> MAIGEFMVSLPRMVYPQPKVLTPCRKDVLVVTPWLAPIVWEGTFNIDILNEQFRLQNTTIGLTVFAIKKYVAFLKLFLETAEKHFMVGHRVHYYVFTDQPAAVPRVTLGTGRQLSVLEVRAYKRWQDVSMRRMEMIS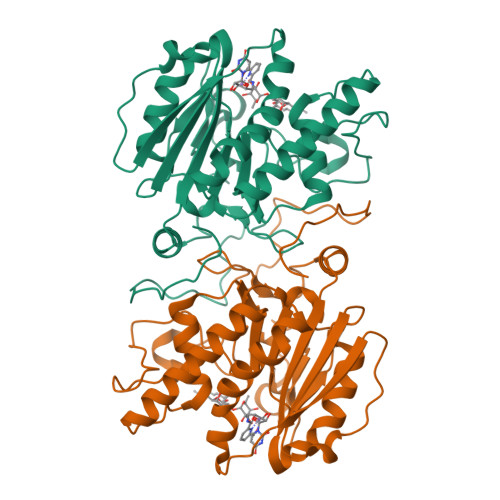DFCERRFLSEVDYLVCVDVDMEFRDHVGVEILTPLFGTLHPGFYGSSREAFTYERRPQSQAYIPKDEGDFYYGGAFFGGSVQEVQRLTRACHQAMMVDQANGIEAVWHDESHLNKYLLRHKPTKVLSPEYLWDQQLLGWPAVLRKLRFTAVPK> GPLGSGQLKVTDVQPAARGSIVDRNNDRLAFTIEARALTFQPKRIRRQLEEARKKTSAAPDPQQRLRDIAQEVAGKLNNKPDAAAVLKKLQSDETFVYLARAVDPAVASAICAKYPEVGAERQDLRQYPGGSL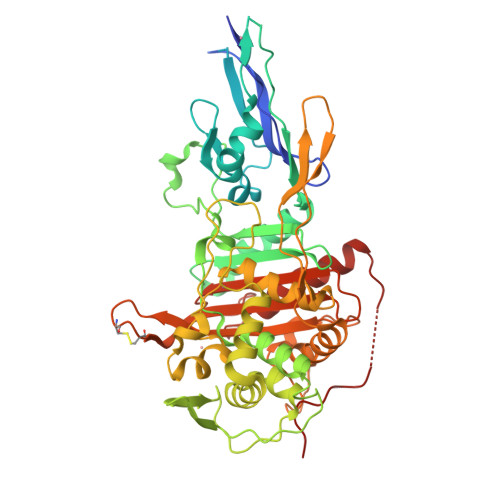AANVVGGIDWDGHGLLGLEDSLDAVLAGTDGSVTYDRGSDGVVIPGSYRNRHKAVHGSTVVLTLDNDIQFYVQQQVQQAKNLSGAHNVSAVVLDAKTGEVLAMANDNTFDPSQDIGRQGDKQLGNPAVSSPFEPGSVNKIVAASAVIEHGLSSPDEVLQVPGSIQMGGVTVHDAWEHGVMPYTTTGVFGKSSNVGTLMLSQRVGPERYYDMLRKFGLGQRTGVGLPGESAGLVPPIDQWSGSTFANLPIGQGLSMTLLQMTGMYQAIANDGVRVPPRIIKATVAPDGSRTEEPRPDDIRVVSAQTAQTVRQMLRAVVQRDPMGYQQGTGPTAGVPGYQMAGKTGTAQQINPGCGCYFDDVYWITFAGIATADNPRYVIGIMLDNPARNSDGAPGHSAAPLFHNIAGWLMQRENVPLSPDPGPPLVLQAT To demonstrate the capabilities of MMQX, the conversion of oxaloacetic acid to phosphoenolpyruvate by phosphoenolpyruvate carboxy­kinase (PEPCK) is observed with a time resolution of 40 ms. Here, millisecond mix-and-quench crystallography (MMQX) has been developed, which yields millisecond time-resolved data using far fewer crystals and routine remote synchrotron data collection. The Ω-loop in all our structures is open and disordered, consistent with the hypothesis that the loop is open in unoccupied active sites as well as during the product-release steps after the reaction is catalyzed.

As the unmixed and Δt ≃ 40 ms data are isomorphous, maps corresponding to F o,mixed − F o,unmixed can be calculated. These show clear hallmarks of GTP to GDP conversion, with relaxation of the α- and β-phosphates away from the Mn2+ catalytic ions [Figs. 2(a) and 2(b)]. As the Δt ≃ 120 ms data are no longer isomorphous to the unmixed data, we cannot use as sensitive a method for analysis, but general inspection of the data suggests that little has changed in the active site between 40 and 120 ms.

> GSMPPQLHNGLDFSAKVIQGSLDSLPQEVRKFVEGNAQLCQPEYIHICDGSEEEYGRLLAHMQEEGVIRKLKKYDNCWLALTDPRDVARIESKTVIITQEQRDTVPIPKSGQSQLGRWMSEEDFEKAFNARFPGCMKGRTMYVIPFSMGPLGSPLAKIGIELTDSPYVVASMRIMTRMGTSVLEALGDGEFIKCLHSVGCPLPLKKPLVNNWACNPELTLIAHLPDRREIISFGSGYGGNSLLGKKCFALRIASRLAKEEGWLAEHMLILGITNPEGKKKYLAAAFPSACGKTNLAMMNPTLPGWKVECVGDDIAWMKFDAQGNLRAINPENGFFGVAPGTSVKTNPNAIKTIQKNTIFTNVAETSDGGVYWEGIDEPLAPGVTITSWKNKEWRPQDEEPCAHPNSRFCTPASQCPIIDPAWESPEGVPIEGIIFGGRRPAGVPLVYEALSWQHGVFVGAAMRSEATAAAEHKGKVIMHDPFAMRPFFGYNFGKYLAHWLSMAHRPAAKLPKIFHVNWFRKDKNGKFLWPGFGENSRVLEWMFGRIEGEDSAKLTPIGYVPKEDALNLKGLGDVNVEELFGISKEFWEKEVEEIDKYLEDQVNADLPYEIERELRALKQRISQM(1R,2R,3R,4R,5S,6S)-6-HYDROXYCYCLOHEXANE-1,2,3,4,5-PENTAYL PENTAKIS[DIHYDROGEN (PHOSPHATE)] | C6 H17 O21 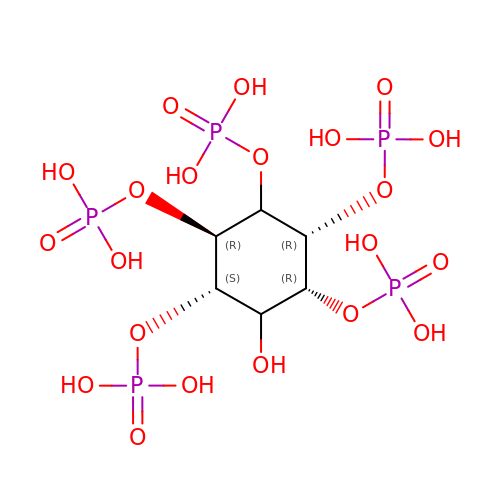P5 | CTPQAXVNYGZUAJ-RTWKJESVSA-N> MKEEVKGIPVRVALRCRPLVSKEIKEGCQTCLSFVPGEPQVVVGNDKSFTYDFVFDPSTEQEEVFNTAVAPLIKGVFKGYNATVLAYGQTGSGKTYSMGGAYTAEQEHDSAI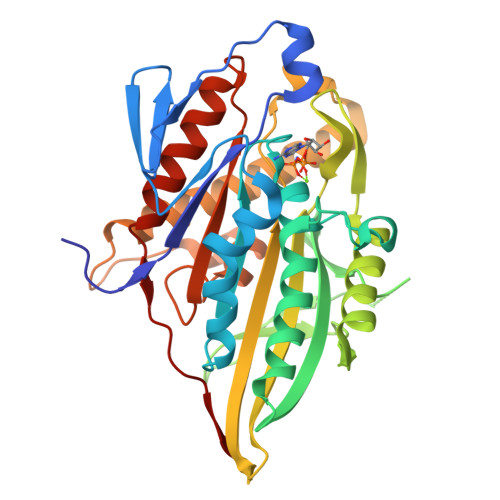GVIPRVIQLLFKEINKKSDFEFTLKVSYLEIYNEEILDLLCSSREKATQINIREDPKEGIKIVGLTEKTVLVASDTVSCLEQGNNSRTVASTAMNSQSSRSHAIFTISIEQRKKNDKNSSFRSKLHLVDLAGSERQKKTKAEGDRLREGININRGLLCLGNVISALGDDKKGNFVPYRDSKLTRLLQDSLGGNSHTLMIACVSPADSNLEETLNTLRYADRARKIKNKPIINHHHHHHH> GIDPFTAKRTHRVINHPYYFPFNGRQAEDYLRSKERGEFVIRQSSRGDDHLVITWKLDKDLFQHIDIQELEKENPLALGKVLIVDNQKYNDLDQIIVEYLQNKVRLLNEMTSSEKFKSGTKKDVVKFIEDYSRVNPNKSVYYFSLNHDNPGWFYLMFKINANSKLYTWNVKLTNTGYFLVNYNYPSVIQLCNGFKTLLKSNSSKNRMNNYR;> ESGLVNADLDVKDELMFSPLVDS

Phosphorylation of CTD residues is thought to recruit multiple co-factors, including the essential and conserved transcription factor Spt6, which directly binds to and co-localizes with RNAPII at sites of transcription. The C-terminal region (residues 1250–1440) comprises a tandem SH2 (tSH2) domain that is tethered to the core by a flexible 21-residue helix and contains both of the two known SH2 structural motifs in yeast. The N-terminal module (nSH2) resembles a canonical SH2 domain while the C-terminal module (cSH2) is vestigial and does not conserve the residues that are normally associated with binding to pY-containing peptides that comprise the vast majority of known SH2 domain ligands. We therefore took an unbiased approach to map the tSH2 domain binding site within RNAPII and, contrary to the earlier assumptions, found that Spt6 tSH2 directly binds the flexible, 86 residue Rpb1 linker (residues 1456–1541) that tethers the heptad CTD repeats to the RNAPII core.

To understand how Spt6 tSH2 preferentially recognizes the Rpb1 linker peptide containing pS1493, we determined a crystal structure of Spt6 tSH2 in complex with Rpb11476-1500 pS1493. The crystals contained one complex in the asymmetric unit. Spt6 residues T1250-R1451 and Rpb1 residues L1479-S1498 were visible in the electron density map. The structure shows the peptide draping over the tSH2 domain in an extended conformation that buries 1,194 Å2 of solvent-accessible surface area with both hydrophobic and polar contacts contributing to the interaction. All of the contacts involve the cSH2 module, and are distant from both the vestigial pY-binding site in the cSH2 module and the canonical pY-binding site of the nSH2 module. The pS1493-binding pocket is formed primarily by Spt6 residues K1355, K1435, and Y1381, with the phosphate moiety forming hydrogen bonding interactions with all three of these side chains. K1435 and Y1381 are strictly conserved among Spt6 homologs, which suggests that the binding geometry is conserved throughout eukaryotes. Rpb1 residues L1479 to F1492 lie against the tSH2 domain in an extended conformation to bury a total of 923 Å2 of solvent-accessible surface area and eight hydrogen bonding interactions. In particular, the side chains of F1492, L1490, and L1484 are buried in a deep hydrophobic groove on the surface of Spt6 tSH2. Mutating either one (Spt6K1435A) or both (Spt6K1355A,K1435A) of the primary phosphate contacts in the binding pocket reduced the affinity for Fl-Rpb11476-1511 pS1493 approximately 100-fold (KD 8.3 μM and 25 μM respectively).> VNLKQAILQAWKERWSDYQWAINMKK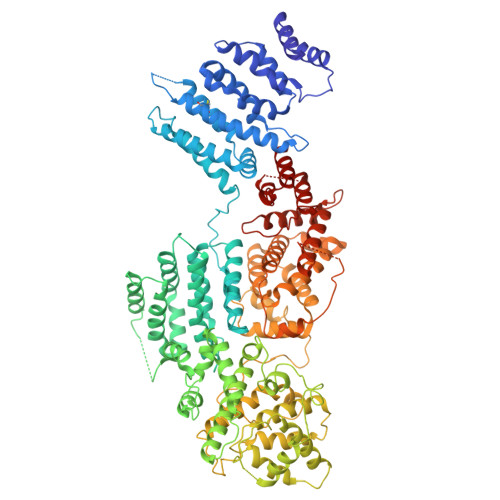FFPKGATWDILNLAEALLEQAMIGPSPNPLILSYLKYAISSQMVSCSSVLTAISKFDDFSRDLCVQALLDIMDMFCDRLSCHGKAEECIGLCRALLSALHWLLRCTAASAERLQEGLEAGTPAPGEKQLALCLQCLEKTLSSTKNRALLHIAKLEEASSWTAIEHSLLKLGEILANLSNPQLRSQAERCGTLIRSIPSMLSVHSEQLHKTGFPTIHALILLEGTMNLTGEMQPLVEQLMMVKRMQHIPTPLFVLEIWKACFVGLIESPEGTQELKWTAFTYLKIPQVLVKLKKYFHGEKDFTEDVNCAFEFLLKLTPLLDKADQRCNCDCTNFLLQECNKQGLLSEVNFASLVGKRTADRDPQLKSSENANIQPNPGLILRAEPTVTNILKTMDADHSKSPEGLLGVLGHMLSGKSLDLLLAAAAATGKLKSFARKFINLNEFTTHGSGESTKTASVRALLFDISFLMLCHVAQTYGSEVILSESSSGEEVPFFETWMQTCMPEEGKILNPDHPCFRPDSTKVESLVALLNNSSEMKLVQMKWHEACLSISAAILEILNAWENGVLAFESIQKITDNIKGKVCSLAVCAVAWLVAHVRMLGLDEREKSLQMIRQLAGPLYSENTLQFYNERVVIMNSILEHMCADVLQQTATQIKFPSTGVDTMPYWNLLPPKRPIKEVLTDIFAKVLEKGWVDSRSIHILDTLLHMGGVYWFCNNLIKELLKETRKEHTLRAVQLLYSIFCLDMQQVTLVLLGHILPGLLTDSSKWHSLMDPPGTALAKLAVWCALSSYSSHKGQASSRQKKRHREDIEDYVSLFPVEDMQPSKLMRLLSSSDDDANILSSPTDRSMNSSLSASQLHTVNMRDPLNRVLANLFLLISSILGSRTAGPHTQFVQWFMEECVGCLEQDSRGSILQFMPFTTVSELVKVSAMSSPKVVLAITDLSLPLGRQVAAKAIA> XXXXXXXXXXXXXXXXXXXXXXXXXXXXXXXXXXXXXXXXXXXXXXXXXXXXXXXXXXXXXXXXXXXXXXXXXXXXXXXXXXXXXXXXXXXXXXXXXXXXXXXXXXXXXXXXXXXXXXXXXXXXXXXXXXXXXXXXXXXXXXXXXXXXXXXXXXXXXXXXXXXXXXXXXXXXXXXXXXXXXXXXXXXXXXXXXXXXXXXXXXXXXXXXXXXXXXXXXXXXXXXXXXXXXXXXXXXXXXXXXXXXXXXXXXXXXXXXXXXXXXXXXXXXXXXXXXXXXXXXXXXXXXXXXXXXXXXXXXXXXXXXXXFSTNFRDTVDILVGWHIDHTQKPSLTQQVSGWLQSLEPFWVADLAFSTTLLGQFLEDMEAYAEDLSHVASGESVDEDVPPPSVSLPKLAALLRVFSTVVRSIGERFSPIRGPPITEAYVTDVLYRVMRCVTAANQVFFSEAVLTAANECVGVLLGSLDPSMTIHCDMVITYGLDQLENCQTCGTDYIISVLNLLTLIVEQINTKLPSSFVEKLFIPSSKLLFLRYHKEKEVVAVAHAVYQAVLSLKNIPVLETAYKLILGEMTCALNNLLHSLQLPEACSEIKHEAFKNHVFNVDNAKFVVIFDLSALTTIGNAKNSLIGMWALSPTVFALLSKNLMIVHSDLAVHFPAIQYAVLYTLYSHCTRHDHFISSSLSSSSPSLFDGAVISTVTTATKKHFSIILNLLGILLKKDNLNQDTRKLLMTWALEAAVLMRKSETYAPLFSLPSFHKFCKGLLANTLVEDVNICLQACSSLHALSSSLPDDLLQRCVDVCRVQLVHSGTRIRQAFGKLLKSIPLDVVLSNNNHTEIQEISLALRSHMSKAPSNTFHPQDFSDVISFILYGNSHRTGKDNWLERLFYSCQRLDKRDQSTIPRNLLKTDAVLWQWAIWEAAQFTVLSKLRTPLGRAQDTFQTIEGIIRSLAAHTLNPDQDVSQWTTADNDEGHGNNQLRLVLLLQYLENLEKLMYNAYEGCANALTSPPKVIRTFFYTNRQTCQDWLTRIRLSIMRVGLLAGQPAVTVRHGFDLLTEMKTTSLSQGNELEVTIMMVVEALCELHCPEAIQGIAVWSSSIVGKNLLWINSVAQQAEGRFEKASVEYQEHLCAMTGVDCCISSFDKSVLTLANAGRNSASPKHSLNGESRKTVLSKPTDSSPEVINYLGNKACECYISIADWAAVQEWQNSIHDLKKSTSSTSLNLKADFNYIKSLSSFESGKFVECTEQLELLPGENINLLAGGSKEKIDMKKLLPNMLSPDPRELQKSIEVQLLRSSVCLATALNPIEQDQKWQSITENVVKYLKQTSRIAIGPLRLSTLTVSQSLPVLSTLQLYCSSALENTVSNRLSTEDCLIPLFSEALRSCKQHDVRPWMQALRYTMYQNQLLEKIKEQTVPIRSHLMELGLTAAKFARKRGNVSLATRLLAQCSEVQLGKTTTAQDLVQHFKKLSTQGQVDEKWGPELDIEKTKLLYTAGQSTHAMEMLSSCAISFCKSVKAEYAVAKSILTLAKWIQAEWKEISGQLKQVYRAQHQQNFTGLSTLSKNILTLIELPSVNTMEEEYPRIESESTVHIGVGEPDFILGQLYHLSSVQAPEVAKSWAALASWAYRWGRKVVDNASXXXXXXXXXXXXXXXXXXXXXXXXXXXXXXXXXXXXXXXXXXXXXXXXXXXXXXXXXXXXXXXXXXXXXXXXXXXXXXXXXXXXXXXXEGVIKVWRKVVDRIFSLYKLSCSAYFTFLKLNAGQIPLDEDDPRLHLSHRVEQSTDDMIVMATLRLLRLLVKHAGELRQYLEHGLETTPTAPWRGIIPQLFSRLNHPEVYVRQSICNLLCRVAQDSPHLILYPAIVGTISLSSESQASGNKFSTAIPTLLGNIQGEELLVSECEGGSPPASQDSNKDEPKSGLNEDQAMMQDCYSKIVDKLSSANPTMVLQVQMLVAELRRVTVLWDELWLGVLLQQHMYVLXXXXXXXXXXXXXXXXXXXXXXXXXXXXXXXXXXXXXXXXXXXXXXXXXXXXXXXXPHEKWFQDNYGDAIENALEKLKXXXXXXXXXXXXXXXXXXXXXXXXXXXXXXXYILRLEEISPWLAAMTNTEIALPGEVSARDTVTIHSVGGTITILPTKTKPKKLLFLGSDGKSYPYLFKGLEDLHLDERIMQFLSIVNTMFATINRQETPRFHARHYSVTPLGTRSGLIQWVDGATPLFGLYKRWQQREAALQAQKAQDSYQTPQNPGIVPRPSELYYSKIGPALKTVGLSLDVSRRDWPLHVMKAVLEELMEATPPNLLAKELWSSCTTPDEWWRVTQSYARSTAVMSMVGYIIGLGDRHLDNVLIDMTTGEVVHIDYNVCFEKGKSLRVPEKVPFRMTQNIETALGVTGVEGVFRLSCEQVLHIMRRGRETLLTLLEAFVYDPLVDWTAGGEAGFAGAVYGGGGQQAESKQSKREMEREITRSLFSSRVAEIKVNWFKNRDEMLVVLPKLDGSLDEYLSLQEQLTDVEKLQGKLLEEIEFLEGAEGVDHPSHTLQHRYSEHTQLQTQQRAVQEAIQVKLNEFEQWITHYQAAFNNLEATQLASLLQEISTQMDLGPPSYVPATAFLQNAGQAHLISQCEQLEGEVGALLQQRRSVLRGCLEQLHHYATVALQYPKAIFQKHRIEQWKTWMEELICNTTVERCQELYRKYEMQYAPQPPPTVCQFITATEMTLQRYAADINSRLIRQVERLKQEAVTVPVCEDQLKEIERCIKVFLHENGEEGSLSLASVIISALCTLTRRNLMMEGAASSAGEQLVDLTSRDGAWFLEELCSMSGNVTCLVQLLKQCHLVPQDLDIPNPMEASETVHLANGVYTSLQELNSNFRQIIFPEALRCLMKGEYTLESMLHELDGLIEQTTDGVPLQTLVESLQAYLRNAAMGLEEETHAHYIDVARLLHAQYGELIQPRNGSVDETPKMSAGQMLLVAFDGMFAQVETAFSLLVEKLNKMEIPIAWRKIDIIREARSTQVNFFDDDNHRQVLEEIFFLKRLQTIKEFFRLCGTFSKTLSGSSSLEDQNTVNGPVQIVNVKTLFRNSCFSEDQMAKPIKAFTADFVRQLLIGLPNQALGLTLCSFISALGVDIIAQVEAKDFGAESKVSVDDLCKKAVEHNIQIGKFSQLVMNRATVLASSYDTAWKKHDLVRRLETSISSCKTSLQRVQLHIAMFQWQHEDLLINRPQAMSVTPPPRSAILTSMKKKLHTLSQIETSIATVQEKLAALESSIEQRLKWAGGANPALAPVLQDFEATIAERRNLVLKESQRASQVTFLCSNIIHFESLRTRTAEALNLDAALFELIKRCQQMCSFASQFNSSVSELELRLLQRVDTGLEHPIGSSEWLLSAHKQLTQDMSTQRAIQTEKEQQIETVCETIQNLVDNIKTVLTGHNRQLGDVKHLLKAMAKDEEAALADGEDVPYENSVRQFLGEYKSWQDNIQTVLFTLVQAMGQVRSQEHVEMLQEITPTLKELKTQSQSIYNNLVSFASPLVTDATNECSSPTSSATYQPSFAAAVRSNTGQKTQPDVMSQNARKLIQKNLATSADTPPSTVPGTGKSVACSPKKAVRDPKTGKAVQERNSYAVSVWKRVKAKLEGRDVDPNRRMSVAEQVDYVIKEATNLDNLAQLYEGWTAWV;> MAGPVSLRDLLMGASAWMGSESPGGSPTEGGGSAAGGPEPPWREDEICVVGIFGKTALRLNSEKFSLVNTVCDRQVFPLFRHQDPGDPGPGIRTEAGAVGEAGGAEDPGAAAGGSVRGSGAVAEGNRTEAGSQDYSLLQAYYSQESKVLYLLLTSICDNSQLLRACRALQSGEAGGGLSLPHAEAHEFWKHQEKLQCLSLLYLFSVCHILLLVHPTCSFDITYDRVFRALDGLRQKVLPLLKTAIKDCPVGKDWKLNCRPCPPRLLFLFQLNGALKVEPPRNQDPAHPDKPKKHSPKRRLQHALEDQIYRIFRKSRVLTNQSINCLFTVPANQAFVYIVPGSQEEDPVGMLLDQLRSHCTVKDPESLLVPAPLSGPRRYQVMRQHSRQQLSFHIDSSSSSSSGQLVDFTLREFLWQHVELVLSKKGFDDSVGRNPQPSHFELPTYQKWISAASKLYEVAIDGKEEDLGSPTGELTSKILSSIKVLEGFLDIDTKFSENRCQKALPMAHSAYQSNLPHNYTMTVHKNQLAQALRVYSQHARGPAFHKYAMQLHEDCYKFWSNGHQLCEERSLTDQHCVHKFHSLPKSGEKPEADRNPPVLYHNSRARSTGACNCGRKQAPRDDPFDIKAANYDFYQLLEEKCCGKLDHINFPVFEPSTPDPAPAKNESSPAPPDSDADKLKEKEPQTQGESTSLSLALSLGQSTDSLGTYPADPQAGGDNPEVHGQVEVKTEKRPNFVDRQASTVEYLPGMLHSNCPKGLLPKFSSWSLVKLGPAKSYNFHTGLDQQGFIPGTNYLMPWDIVIRTRAEDEGDLDTNSWPAPNKAIPGKRSAVVMGRGRRRDDIARAFVGFEYEDSRGRRFMCSGPDKVMKVMGSGPKESALKALNSDMPLYILSSSQGRGLKPHYAQLMRLFVVVPDAPLQIILMPQVQPGPPPCPVFYPEKQEITLPPDGLWVLRFPYAYVTERGPCFPPKENVQLMSYKVLRGVLKAVTQ;> MSESGHSQPGLYGIERRRRWKEPGSGGPQNLSGPGGRERDYIAPWERERRDASEETSTSVMQKTPIILSKPPAERSKQPPPPTAPAAPPAPAPLEKPIVLMKPREEGKGPVAVTGASTPEGTAPPPPAAPAPPKGEKEGQRPTQPVYQIQNRGMGTAAPAAMDPVVGQAKLLPPERMKHSIKLVDDQMNWCDSAIEYLLDQTDVLVVGVLGLQGTGKSMVMSLLSANTPEEDQRTYVFRAQSAEMKERGGNQTSGIDFFITQERIVFLDTQPILSPSILDHLINNDRKLPPEYNLPHTYVEMQSLQIAAFLFTVCHVVIVVQDWFTDLSLYRFLQTAEMVKPSTPSPSHESSSSSGSDEGTEYYPHLVFLQNKARREDFCPRKLRQMHLMIDQLMAHSHLRYKGTLSMLQCNVFPGLPPDFLDSEVNLFLVPFMDSEAESENPPRAGPGSSPLFSLLPGYRGHPSFQSLVSKLRSQVMSMARPQLSHTILTEKNWFHYAARIWDGVRKSSALAEYSRLLA

The PI3K-related kinase (PIKK) SMG1 monitors the progression of metazoan nonsense-mediated mRNA decay (NMD) by phosphorylating the RNA helicase UPF1. SMG1 is a member of the phosphatidylinositol-3-kinase-related kinase (PIKK) family, which also includes the ATM, ATR, DNA-PKc, and mTOR kinases. Despite the confounding name reflecting a possible evolutionary origin with a lipid kinase, and in retrospect the ability of some PIKK family members to bind inositol-6-phosphate, all active PIKKs are Ser-Thr protein kinases. These large, multidomain enzymes share an overall similar architecture: a C-terminal catalytic module (comprising the so-called FAT, kinase, and FATC domains) and an N-terminal α-solenoid (that typically serves as a protein-protein interaction module). SMG8 and SMG9 form an unusual G-domain heterodimer.

To understand the molecular basis for the SMG1i mode of action, we reconstituted purified wild-type SMG1-8-9 with an excess of SMG1i and subjected the sample to single-particle cryo-EM analysis. The resulting reconstruction reached an overall resolution of 3.1 Å, and we observed clear density for the SMG1 inhibitor bound to the kinase active site (Figure 2—figure supplements 1 and 2 and Figure 2—figure supplement 3B). Superposition with our previously published AMPPNP- and substrate-bound model revealed that SMG1i exploits essentially the same binding site as the ATP analog. However, SMG1i wedges deeper in between the N- and C-lobe of the kinase domain and is engaged in more extensive interactions. These observations identify SMG1i as a potent ATP-competitive inhibitor. In the reconstruction of the SMG1i-bound SMG1-8-9 complex, we observed additional density near the end of the kinase domain, protruding from the position where the insertion domain is expected to start. While the lower resolution for this part of the map was not sufficient to unambiguously build an atomic model, this density clearly docks at the substrate-binding site of the kinase domain. Superposition with the previous cryo-EM structure of SMG1-8-9 complex bound to a UPF1 peptide revealed that the additional density in the current reconstruction is mutually exclusive with the position of a bound substrate. We concluded that the SMG1 insertion domain contains a PRD that can directly occupy and block the substrate-binding path in the kinase active site, analogous to other PIKKs. The SMG1 PRD would have to re-arrange upon substrate binding, as observed in the case of the inactive-to-active transition of DNA-PK.>[2x]MGSS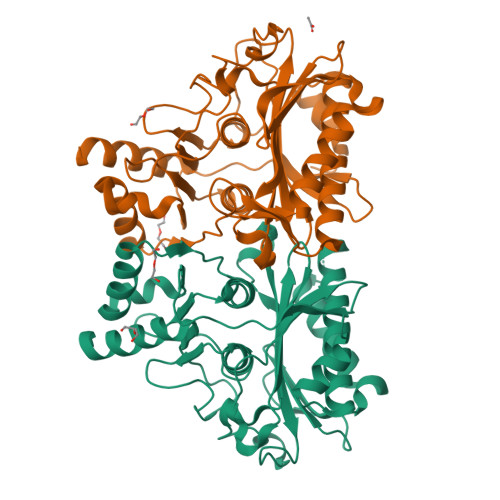HHHHHHENLYFQGMESPSALPSLDQLLKEQGADQTLTDLILAILDRCGKIASALQGTSVDKVGSVNEFGDEQLTVDVIAENLLRSWAQSSEGSAVRAVCSEEDIHLQECHKNGEFILCWDPLDGSSIIDCNWAVGSIVSIWRIGHHGVQWQGADTLIQKTGRQQVASLIVVYGPRTTGVVAVNVDAGGIVKEGTALDLEMKDNGKFICRGKPIIKPQAKIFSPANLRAAQDLPAYKQLIEFWMEKRYTLRYTGGLVPDVYQIFVKQQGVFCNPASKAAPAKLRMCFEVLAIALVVEAAGGRTSNGQKSLLDVAIEHMDHRSALCCGSADEIKRMEETFAALSG>[6x]AGPQLDVSCFAHDKNIGSRTEQLSVVHVASAQDCMKECQALP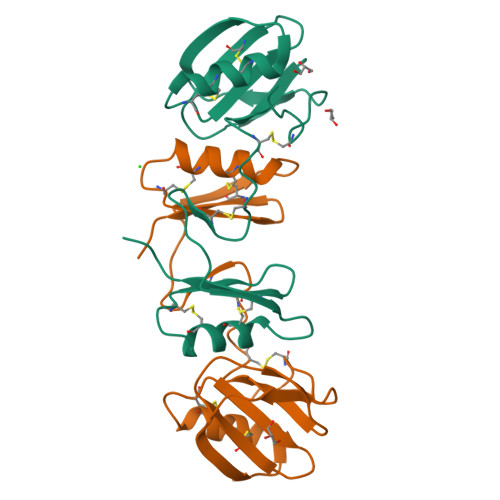TCSHFTYNKNSKKCHLKAGAPEFYTYTGDMTGPRSCEHNCSDACWMDGNNPLAVWDYSGQPPALCWAACMGTPGCDLYTFQGMTCKLYSQTSSKRA Unlike many bacteria, Agrobacterium harbors another redox-associated LTTR, called LsrB (LysR-type symbiosis regulator B). LsrB is solely found in Rhizobiales, such as the plant symbiont Sinorhizobium meliloti or the intracellular mammalian pathogen Brucella abortus (there designated as VtlR = virulence-associated transcriptional LysR-family regulator). LsrB is a major regulator of various cellular responses, including the coordinated regulation of small RNAs, ABC transporter or β-lactam resistance genes. Agrobacterium tumefaciens LsrB possesses four cysteine residues potentially involved in redox sensing.

To experimentally support the biocomputational structure model, we employed cryo-EM of purified LsrB. Instead of the expected tetramers, we captured LsrB dimers, likely due to unstable homotetrameric oligomerization in the absence of DNA. We excluded the DNA-binding domain from our analysis due to its high flexibility, prior to refining the volume density map (resolution 3.9 Å) and fitting it with the AlphaFold 3-generated model. The results show that AlphaFold accurately predicted both (i) the dimeric interface of the two LsrB monomers and (ii) the spatial arrangement of the chains. Based on the validated 3D structure, we were able to localize the two pairs of cysteine residues (C144/C273 and C236/C244). We calculated the distances between the cysteine residues in each pair and found them to be below 10 Å. The cryo-EM structure, combined with structural modeling, provides compelling evidence for the formation of intramolecular disulfide bonds involving both conserved (C144–C273) and nonconserved (C236–C244) cysteine residues. Additionally, the predicted spatial separation of over 50 Å between cysteine residues from different monomers strongly argues against the possibility of intermolecular disulfide bond formation. In contrast, substitution of C273 led to increased H2O2 sensitivity reminiscent of the lsrB-deletion mutant phenotype. When LsrB was reduced with TCEP, which breaks the S-S bond and converts the cysteine residues back to their reduced form (-SH), and subsequently subjected to modification of cysteines with MMTS, which “traps” free thiol groups by forming mixed disulfides, peptides containing all four cysteine residues (C144, C236, C244, C273) were identified with MMTS modification.

>MAMPLDWDKLRIFHAAAEAGSFTHAADKLHLSQSAISRQVSALEQDVGVKLFHRHARGLILTEQGELLYRTAHDVLLKLETVKMQLTETTEKPSGKLRVTTTVGLGQGWLTDKVQEFLQLYPEMSIQLILDNEELDVNMRHADCAIRLRQPQQSDLIQRKLFTVHMHVYAAPSYINRHGEPQSVEDLDNHRIISFGEPAPNYLLDVNWLENAGRSSDNTRIPHLQINSQTSIKRACLLGIGIACLPDYIVGRDPGLIQLSLAADIPSFDTYFCYPDEMKNAAKLKAFRDFIVAKARNWNFGTSAWSHPQFEK[2x]D-allothreonine | C4 H9 N O3 | 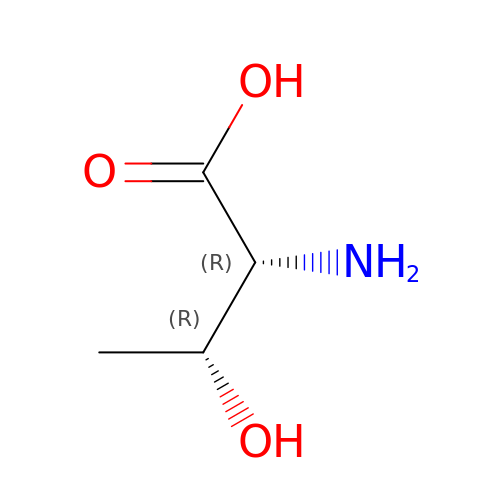AYFVYJQAPQTCCC-PWNYCUMCSA-N> MEQTQKLKLNLQHFASNNVKPQVFNPDNVMMHEKKDGTLMNEFTTPILQEVMENSKIMQLGKYEPMEGTEKKF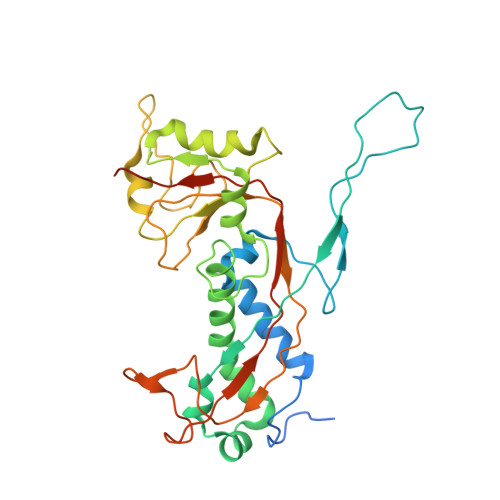TFWADKPGAYWVGEGQKIETSKATWVNATMRAFKLGVILPVTKEFLNYTYSQFFEEMKPMIAEAFYKKFDEAGILNQGNNPFGKSIAQSIEKTNKVIKGDFTQDNIIDLEALLEDDELEANAFISKTQNRSLLRKIVDPETKERIYDRNSDSLDGLPVVNLKSSNLKRGELITGDFDKLIYGIPQLIEYKIDETAQLSTVKNEDGTPVNLFEQDMVALRATMHVALHIADDKAFAKLVPADKRTDSVPGEV>[2x]MAESASKAAPGERVVIGITFGNSNSSIAHTVDDKAEVIANEDGDRQIPTI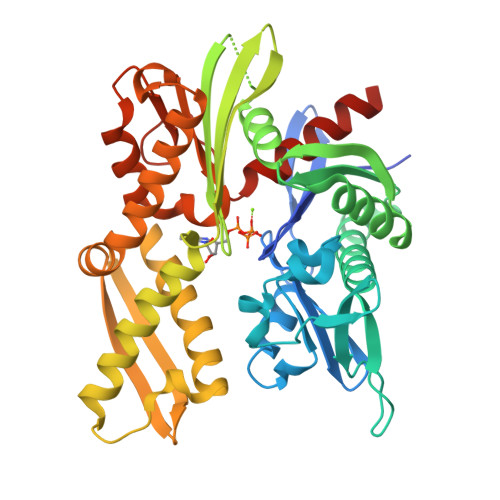LSYVDGDEYYGQQAKNFLVRNPKNTVAYFRDILGQDFKSVDPTHNHASAHPQEAGDNVVFTIKDKAEEDAEPSTLTVSEIATRYLRRLVGAASEYLGKKVTSAVITIPTNFTEKQKAALIAAAAAADLEVLQLISEPAAAVLAYDARPEATISDKIIVVADLGGSRSDVTVLASRSGMYTILATVHDYEYHGIALDKVLIDHFSKEFLKKNPGAKDPRENPRSLAKLRLEAESTKRALSRSTNASFSVESLIDGLDFASTINRLRYETIARTVFEGFNRLVESAVKKAGLDPLDVDEVIMSGGTSNTPRIAANFRYIFPESTRILAPSTDPSALNPSELQARGAALQASLIQEHHHHHH>MGSDKIHHHHHHMKEGTGMVVRSSEITPERISNMRGGKGEVEM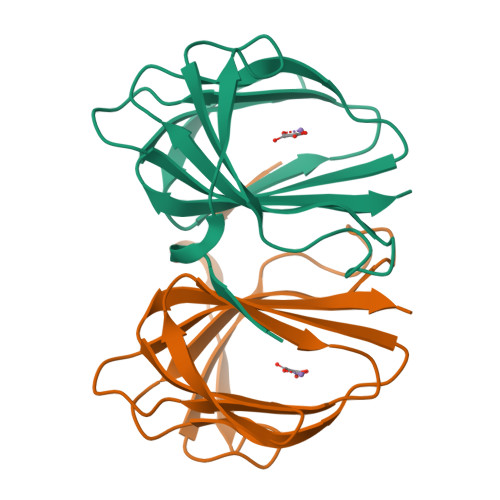AHLLSKEAMHNKARLFARMKLPPGSSVGLHKHEGEFEIYYILLGEGVFHDNGKDVPIKAGDVCFTDSGESHSIENTGNTDLEFLAVIILL[2x]>KEVENQQKLANVVILATGGTIAGAGASAANSATYQAAKVGVDKLIAGVPELADLANVRGEQVMQIASESITNDDLLKLGKRVAELADSNDVDGIVITHGTDTLEETAYFLNLVQKTDKPIVVVGSMRPGTAMSADGMLNLYNAVAVASNKDSRGKGVLVTMNDEIQSGRDVSKSINIKTEAFKSAWGPLGMVVEGKSYWFRLPAKRHTVNSEFDIKQISSLPQV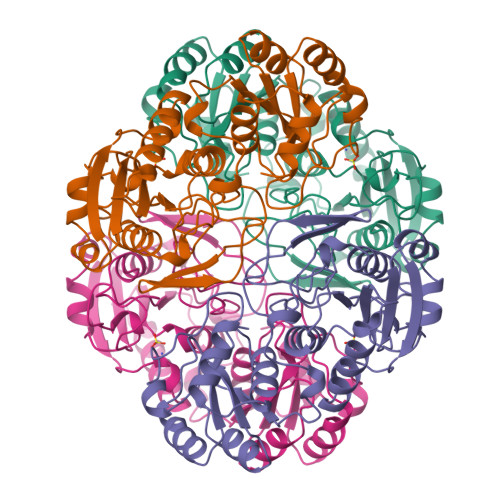DIAYSYGNVTDTAYKALAQNGAKALIHAGTGNGSVSSRVVPALQQLRKNGTQIIRSSHVNQGGFVLRNAEQPDDKNDWVVAHDLNPEKARILAMVAMTKTQDSKELQRIFWEY[2x]>[4x]GAMGLEKDFKRYGDALKPDTSVPGKSKDIRTTKDFLNGYKNDHAKEIVDGFRSDMSIKQLVDLFVKGSWSAEQKGALAWEIESRALKVTFQNKSEKYNRLFREIASAGVVDAKATEQLAPQLMLLNLSNDGFGGRSDPLSKLVLVAKQLENDGQVGVARQLLEKMYSAAAVLSNPTLYSDSENANASKLLSSLAAIHAKNPMHDTSM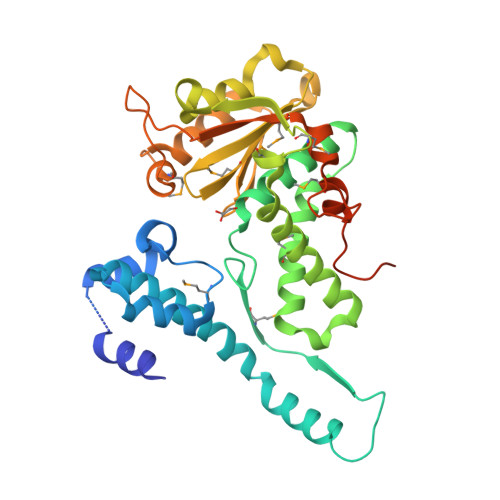KVWQEKLEGKQALTVNGVVEKITDASANGKPVLLELDAPGHAMAAWAKGSGDDRVYGFYDPNAGIVEFSSAEKFGDYLTRFFGKSDLNMAQSYKLGKNDAGEAIFNRVVVMDGNTLASYKPTFGDKTTMQGILDLPVFDATPMKKPGTSDVDGNAKAVDDTKEA>[3x]MAAQGFLLIATFLL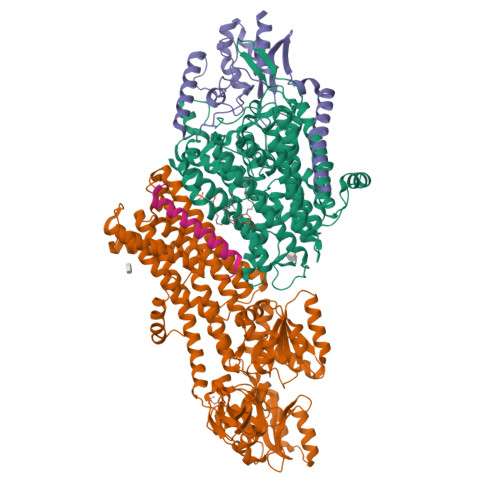VLMVLARPLGSGLARLINDIPLPGTTGVERVLFRALGVSDREMNWKQYLCAILGLNMLGLAVLFFMLLGQHYLPLNPQQLPGLSWDLALNTAVSFVTNTNWRSYSGETTLSYFSQMAGLTVQNFLSAASGIAVIFALIRAFTRQSMSTLGNAWVDLLRITLWVLVPVALLIALFFIQQGALQNFLPYQAVNTVEGAQQLLPMGPVASQEAIKMLGTNGGGFFNANSSHPFENPTALTNFVQMLAIFLIPTALCFAFGEVMGDRRQGRMLLWAMSVIFVICVGVVMWAEVQGNPHLLALGTDSSINMEGKESRFGVLVSSLFAVVTTAASCGAVIAMHDSFTALGGMVPMWLMQIGEVVFGGVGSGLYGMMLFVLLAVFIAGLMIGRTPEYLGKKIDVREMKLTALAILVTPTLVLMGAALAMMTDAGRSAMLNPGPHGFSEVLYAVSSAANNNGSAFAGLSANSPFWNCLLAFCMFVGRFGVIIPVMAIAGSLVSKKSQAASSGTLPTHGPLFVGLLIGTVLLVGALTFIPALALGPVAEYLS;>FEPTLVVQALKEAVKKLNPQAQWRNPVMFIVWIGSLLTTCISIAMASGAMPGNALFSAAISGWLWITVLFANFAEALAEGRSKAQANSLKGVKKTAFARKLREPKYGAAADKVPADQLRKGDIVLVEAGDIIPCDGEVIEGGASVDESAITGESAPVIRESGGDFASVTGGTRILSDWLVIECSVNPGETFLDRMIAMVEGAQRRKTPNEIALTILLIALTIVFLLATATLWPFSAWGGNAVSVTVLVALLVCLIPTTIGGLLSAIGVAGMSRMLGANVIATSGRAVEAAGDVDVLLLDKTGTITLGNRQASEFIPAQGVDEKTLADAAQLASLADETPEGRSIVILAKQRFNLRERDVQSLHATFVPFTAQSRMSGINIDNRMIRKGSVDAIRRHVEANGGHFPTDVDQKVDQVARQGATPLVVVEGSRVLGVIALKDIVKGGIKERFAQLRKMGIKTVMITGDNRLTAAAIAAEAGVDDFLAEATPEAKLALIRQYQAEGRLVAMTGDGTNDAPALAQADVAVAMNSGTQAAKEAGNMVDLDSNPTKLIEVVHIGKQMLMTRGSLTTFSIANDVAKYFAIIPAAFAATYPQLNALNIMCLHSPDSAILSAVIFNALIIVFLIPLALKGVSYKPLTASAMLRRNLWIYGLGGLLVPFIGIKVIDLLLTVCGLV[3x];>LRPALSTFIFLLLITGGVYPLLTTVLGQWWFPWQANGSLIREGDTVRGSALIGQNFTGNGYFHGRPSATAEMPYNPQASGGSNLAVSNPELDKLIAARVAALRAANPDASASVPVELVTASASGLDNNITPQAAAWQIPRVAKARNLSVEQLTQLIAKYSQQPLVKYIGQPVVNIVELNLALDKLDE[3x];>[3x]MSAGVITGVLLVFLLLGYLVYALINAE> MKKHHHHHHDNATDDPVDLVYAAEKIIQKRVKKGVVEYRVKWKGWNQRYNTWEPEVNILDRRLIDIYEQ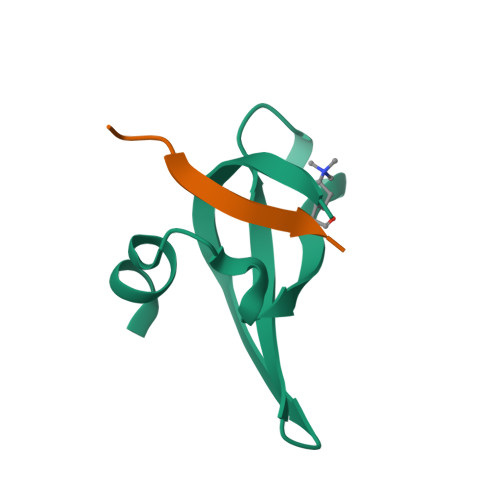TNK;> APRKQLATKAARKSAPST> MGHHHHHHSGIALSRLAQERRAWRKDHPFGFVAVPTKNPDG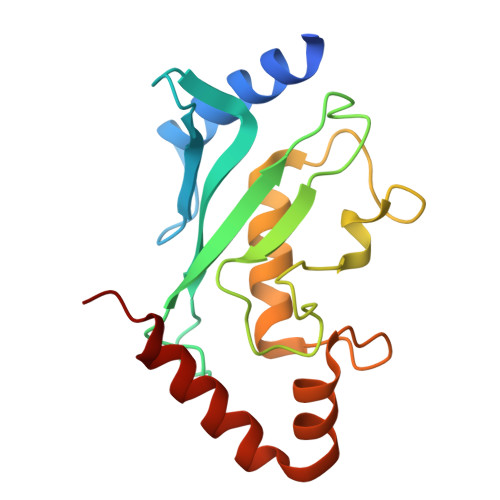TMNLMNWECAIPGKKGTPWEGGLFKLRMLFKDDYPSSPPKCKFEPPLFHPNVYPSGTVCLSILEEDKDWRPAITIKQILLGIQELLNEPNIQDPKQAEAYTIYCQNRVEYEKRVRAQAKKFAPS> KVLKISQTKYEEILKISKKYIFINQVDKSFHEAVDDLNQQDFIAVSGDGANMGRKCKMPFLVLSTDHQIYIFDIQVMQYHAFESGLKKILEGDSPKKIAHDCRKLSDCLYHKHNVKLKSVFDTQVGDLIITKNKKVTLPNKVKSLGECLTNYLGLQQNTIDEKLDIVQSTERPLSVKIKDSLARNIAFL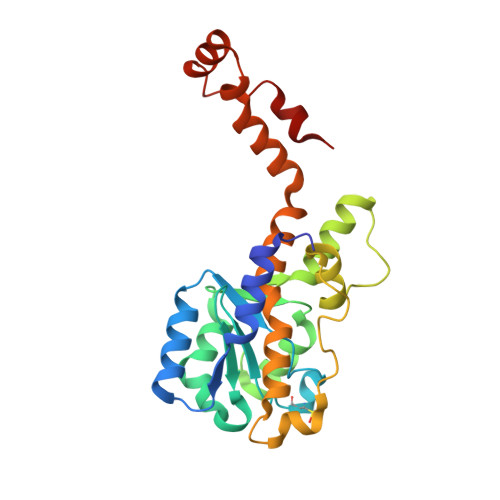HHLSEVINEEMQLPFYRGVECYIENIRSSDDFKAWELCGKLNQIPKEFRNAIDY>[2x]MNFSPREIVSELDRFIIGQKDAKRAVAIALRNRWRRQQLEGQMREEVMPKNILMIGPTGVGKTEISRRLAKLAGAPFVKVEATKFTEVGYVGRDVEQIIRDLVEIAITLVREKRREDVKAKAHLNAEERVLDALVGKTASPATRDSFRKKLRNGEMDDKEIEIEVSDSGASPNFEIPGMPGANIGVLNISDMLGKA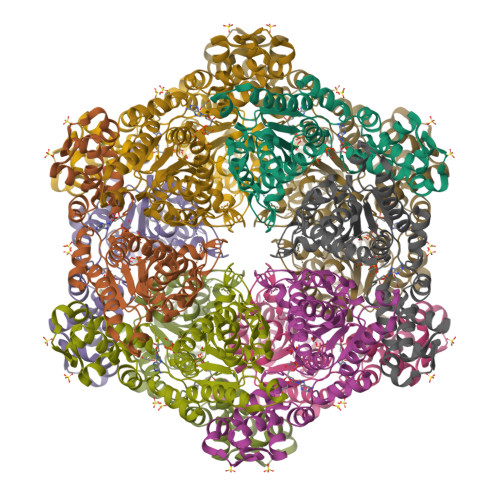MGGRTKTRKTTVKDSYPILINDESDKLLDQDQIVQEALRVSEDEGIVFIDEIDKIAAREGGSGAGVSREGVQRDLLPLVEGTTVATKYGPVKTDHILFITSGAFHVSKPSDLLPELQGRLPIRVELSALTREDFRRILTETEASLIKQYIALMETEEVKLEFSDDAIDALADIAVDLNATVENIGARRLQTVIEKVLDEISFTAPDKAGATFIIDAAYVKEGHHHHHH>[2x]MEDGAQMRVVAFGDQTYDCSEAVSQLLRVRDDAIVVDFLERAPAVLKAELARLSSEQQEETPRFATLAELVPRYRAGTLNPAVSQALTCIAQLGLFIRQHSSGQEAYPTAHDSCITGVATGALTAVAVGSASSVTALVPLALHTVAVAVRLGARAWEIGSCLADARRGANGRYASWTSAVGGISPQDLQDRISAYTAEQALASVSVPYLSAAVGPGQSSVSAAPVILDAFLSTLLRPLTTTRLPITAPYHAPHLFTAKDVQHVTDCLPPSEAWPTVRIPIISFSRDEAVSRGASFPAAMSEAVRDCLIRPIALDRMAVSIANHARDLGKDSVLPSPIALSFSDK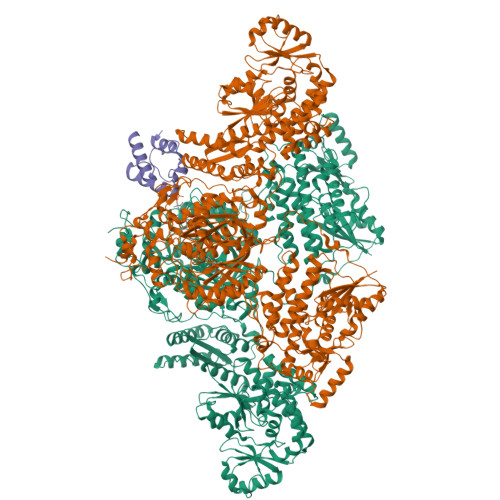LGPQVNSHLPGAKAPTPELTSKSIPSAIGAEQQPMAKSPIAILAASGRFPQSSSMDQFWDVLINGVDTHELVPPTRWNAATHVSEDPKAKNVSGTGFGCWLHEAGEFDAAYFNMSPREAPQVDPAQRLALLTATEALEQAGVVPNRTSSTQKNRVGVWYGATSNDWMETNSAQNVDTYFIPGGNRAFIPGRVNYFHKFSGPSYTIDTACSSSLAALHMACNALWRGEVDTAIVGGTNVLTNPDMTAGLDAGHFLSRSGNCKTFDDEADGYCRGEAVVTLILKRLPDAQADKDPIQASILGIATNHSAEAASITRPHAGAQQDLFQQVLTETGLTANDISVCEMHGTGTQAGDSGETTSVVETLAPLNRSGSAVRTTPLYIGAVKSNVGHAESAAGVSSLAKILLMLKHSKIPPHVGIKTKLNHRLPDLAARNTHIARSEVPWPRPKNGKRRVLLNNFSAAGGNTCLVLEDAPEPEDSQEVDPREHHIVALSAKTPDSMVNNLTNMITWIDKHSGDSLATLPQLSYTTTARRVHHRHRAVATGTDLLQIRSSLQEQLDRRVSGERSIPHPPNGPSFVLAFTGQGSAFAGMGVDLYKRFASFRSDIARYDQICEGMSLPSIKAMFEDEKVFSTASPTLQQLTHVCFQMALYRLWKSLGVQAKAVVGHALGEYAALYAAGVLSQSDTLYLVGRRAQLMEKHLSQGTHAMLAVRAKEEAIVAAIDGPPGEAYEFSCRNGEQRNVLGGTVAQIQAAKAALEAKKIRCQYLDTPMAFHTGQVDPILPELLQVAAACSIQDPQIPVISPAYGKVIRSAKDFQPEYFTHHCRSSVNMVDALQSAVEEGLLDKNVIGLEIGPGPVVTQFVKEAVGTTMQTFASINKDKDTWQLMTQALAKFYLAGASVEWSRYHEDFPGAQKVLELPAYGWALKNYWLQYVNDWSLRKGDPAVVVAASAAALEHHHHHH;> GSHMDPSPNEIGTVWRDALKILSEESGLTDEELTDDTSFADVGVDSLMSLVITSRLRDELDIDFPDRALFEECQTIFDLRKRFSGSTE> SSDTRKHKFDTSTWA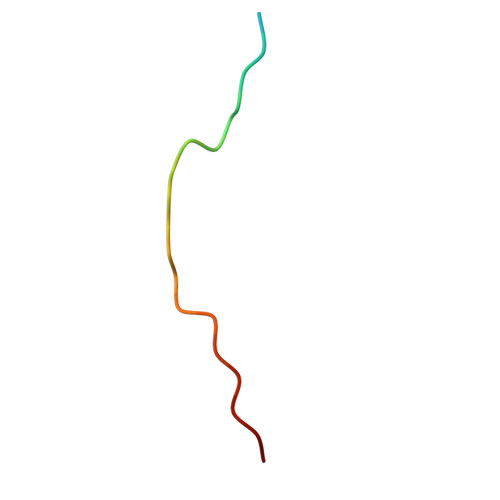LPNKRRRI>[2x]IQTTAPPVKESSFVEKMKKTGRNIIVFYGSQTGTAEEFANRLSKDAHRYGMRGMSADPEEYDLADLSSLPEIDKSLVVFCMATYGEGDPTDNAQDFYDWLQETDVDLTGVKFAVFGLGNKTYEHFNA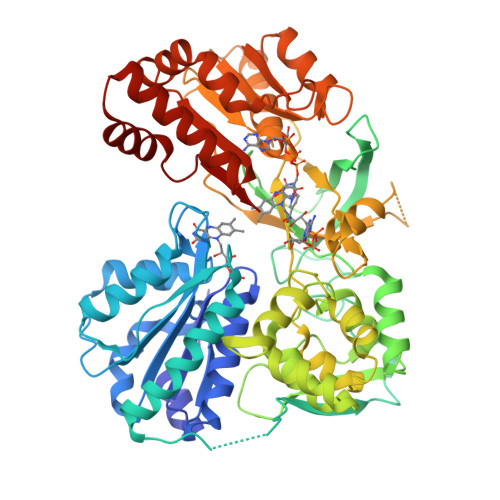MGKYVDQRLEQLGAQRIFELGLGDDDGNLEEDFITWREQFWPAVCEFFGVEATGEESSIRQYELVVHEDMDVAKVYTGEMGRLKSYENQKPPFDAKNPFLAAVTANRKLNQGTERHLMHLELDISDSKIRYESGDHVAVYPANDSALVNQIGEILGADLDVIMSLNNLDEESNKKHPFPCPTTYRTALTYYLDITNPPRTNVLYELAQYASEPSEQEHLHKMASSSGEGKELYLSWVVEARRHILAILQDYPSLRPPIDHLCELLPRLQARYYSIASSSKVHPNSVHICAVAVEYEAKSGRVNKGVATSWLRAKEPAGENGGRALVPMFVRKSQFRLPFKSTTPVIMVGPGTGIAPFMGFIQERAWLREQGKEVGETLLYYGCRRSDEDYLYREELARFHKDGALTQLNVAFSREQAHKVYVQHLLKRDREHLWKLIHEGGAHIYVCGDARNMAKDVQNTFYDIVAEFGPMEHTQAVDYVKKLMTKGRYSLWS> MESLPVIAAPSMWTRPQIKDFKEKIQQDADSVITVGRGEVVTVRVPTHEEGSYLFWEFATDNYDIGFGVYFEWTDSPNTAVSVHVSESSDDDEEEEENIGCEEKAKK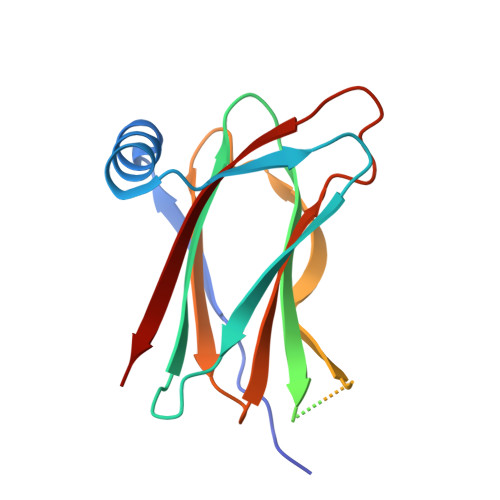NANKPLLDEIVPVYRRDCHEEVYAGSHQYPGRGVYLLKFDNSYSLWRSKSVYYRVYYTR>GGYLLGS[2x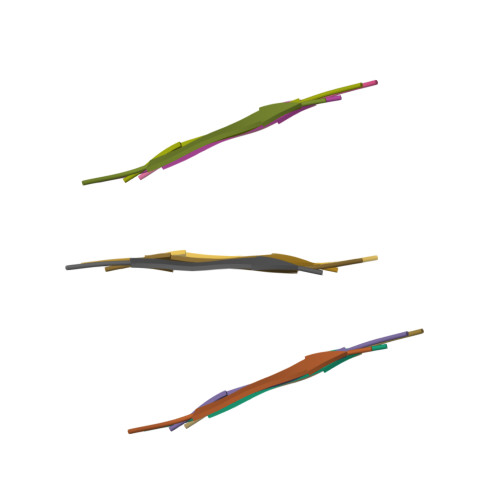]>[3x]MVRERTFIAVKPDGVQRGLIGEIIKRFEAKGFKLAGMKYIQASEDLLKQHYIDLADKPFYPGLCKYMSSGPVVAMCWEGTGVVKTARVMMGETRPADSKPGTIRGDFCIEVGRNIIHG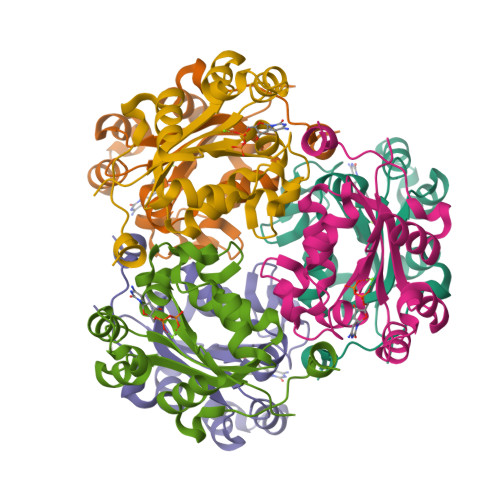SDSVESANKEIALWFKPEELVSWTQTNESWIYE> LPNPLVHLDISIGGRDAGRMVFQLFADTHPITAENFRCLCTGETGLGYWMRPRWYKSTPFHRIVPGFMCQGGDIHRGDGRGGECIYGQ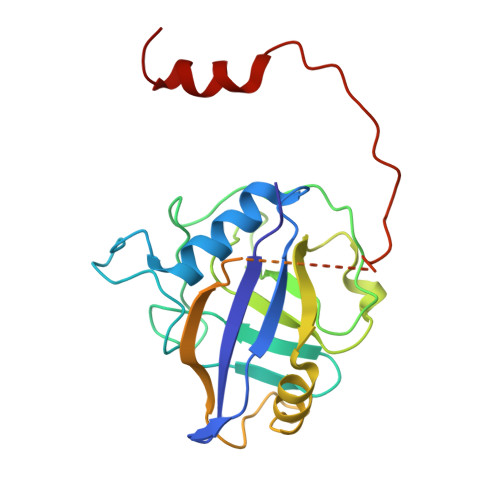FFRDERFLYKHSKRGLLSMAKARRQHTNNSQFFITFDACPWLDGEHVVFGQLQSGAEVLDQIEEQGTPGGWRKRPVEIWNCGELLLNTLREIPREAPAAVRHQEMLKDLIIDATERPEKLYEPSEQVIPIPDDVYIKARRGF>[2x]MSQLAHNLTLSIFDPVANYRAARIICTIGPSTQSVEALKGLIQSGMSVARMNFSHGSHEYH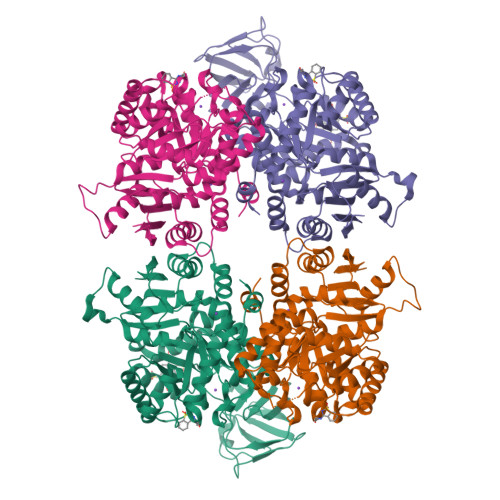QTTINNVRQAAAELGVNIAIALDTKGPEIRTGQFVGGDAVMERGATCYVTTDPAFADKGTKDKFYIDYQNLSKVVRPGNYIYIDDGILILQVQSHEDEQTLECTVTNSHTISDRRGVNLPGCDVDLPAVSAKDRVDLQFGVEQGVDMIFASFIRSAEQVGDVRKALGPKGRDIMIICKIENHQGVQNIDSIIEESDGIMVARGDLGVEIPAEKVVVAQKILISKCNVAGKPVICATQMLESMTYNPRPTRAEVSDVANAVFNGADCVMLSGETAKGKYPNEVVQYMARICLEAQSALNEYVFFNSIKKLQHIPMSADEAVCSSAVNSVYETKAKAMVVLSNTGRSARLVAKYRPNCPIVCVTTRLQTCRQLNITQGVESVFFDADKLGHDEGKEHRVAAGVEFAKSKGYVQTGDYCVVIHADHKVKGYANQTRILLVE>[4x]GHMSELRILRAVDYPRMPWKNGAGSTEEIARDGGDGLDGFGWR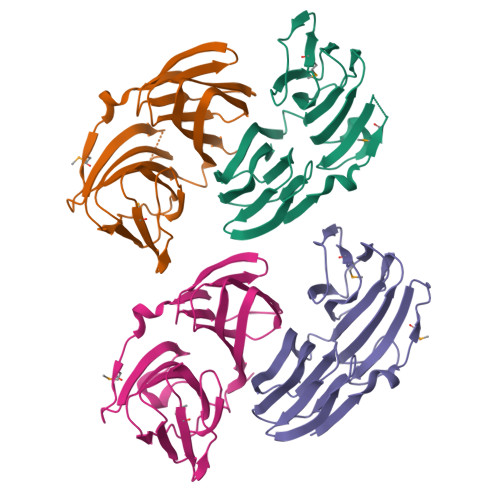LSIADVGESGGFSGFAGYQRIISVLEGGGMRLRVDGAESAPLRARQAFAFSGDSEVHCTLLDGAIRDFNLIYAPRRHRARLQWLRVEGELDWHGTASTLLLFAQQDGVAISLQGQPRGQLAAHDCLCAEGLQGLQHWRLTAHEPAWVCAVELDSLGS>[2x]MASWSHPQFEKGADDDDKVPRGSASLRANDAPIVLLHGFTGWGREEMFGFKYWGGVRGDIEQWLNDNGYRTYTLAVGPLSSNWDRACEAYAQLVGGTVDYGAAHAAKHGHARFGRTYPGLLPELKRGGRIHIIAHSQGGQTARMLVSLLENGSQEEREYAKAHNVSLSPLFEGGHHFVLSVTTIATPHDGTTLV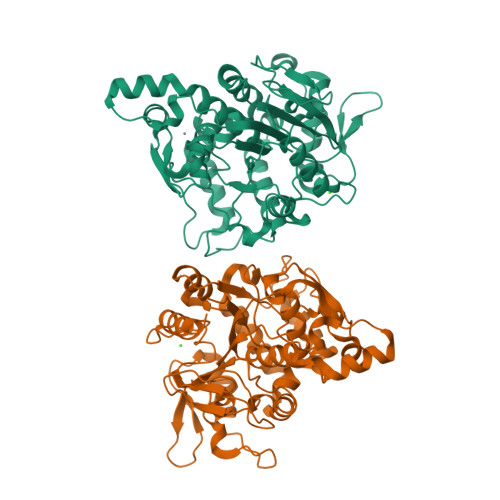NMVDFTDRFFDLQKAVLEAAAVASNVPYTSQVYDFKLDQWGLRRQPGESFDHYFERLKRSPVWTSTDTARYDLSVSGAEKLNQWVQASPNTYYLSFSTERTYRGALTGNHYPELGMNAFSAVVCAPFLGSYRNPTLGIDDRWLENDGIVNTVSMNGPKRGSSDRIVPYDGTLKKGVWNDMGTYNVDHLEIIGVDPNPSFDIRAFYLRLAEQLASLRPPGFSSISAHHHHHHHHHH> MKYDGSKLRIGILHARWNLEIIAALVAGAIKRLQEFGVKAENIIIETVPGSFELPYGSKLFVEKQKRLGKPLDAIIPIGVLIKGSTMHFEYICDSTTHQLMKLNFELGIPVIFGV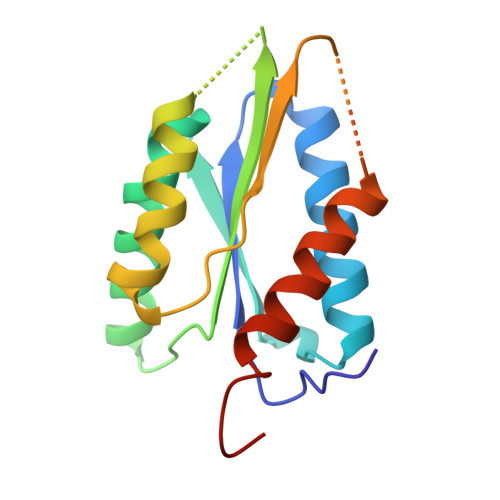LTCLTDEQAEARAGLIEGKMHNHGEDWGAAAVEMATKFNLEHHHHHH> MPRLIKDRVPTPERSVGERVRDFGEVNLGYSWELALREAERCLQCPVEYAPCIKGCPVHINIPGFIKALRENRDNPSKAVREALRIIWRDNTLPAITGRVCPQEEQCEGACVVGKVGDPINIGKLERFVADYAREHGIDDELLLEEIKGIKRNGKKVAIIGAGPAGLTCAADLAKMGYEVTIYEALHQPGGVLIYGIPEFRLPKEIVKKELENLRRLGVKIETNVLVGKTITFEELREEYDAIFIGTGAGTPRIYPWPGVNLNGIYSANEFLTRINLMKAYKFPEYDTPIKVGKRVAVIGGGNTAMDAARSALRLGAEVWILYRRTRKEMTAREEEIKHAEEEGVKFMFLVTPKRFIGDENGNLKAIELEKMKLGEPDESGRRRPIPTGETFIM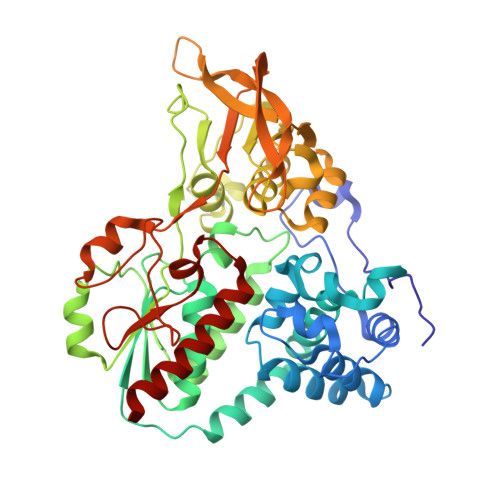EFDTAIIAIGQTPNKTFLETVPGLKVDEWGRIVVDENLMTSIPGVFAGGDAIRGEATVILAMGDGRKAAKAIHQYLSKEK>[2x]MALDLTGYLDRINYRGATDPTLDVLRDLVSAH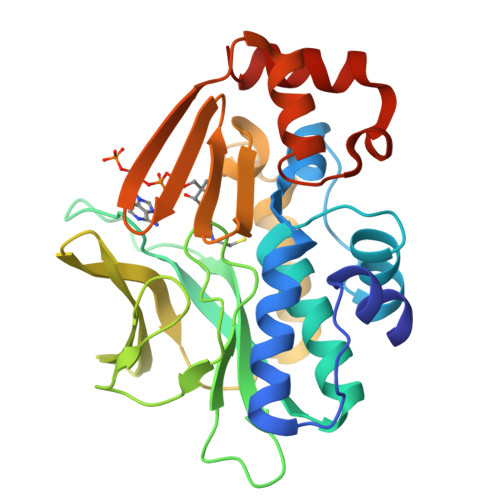TGAIAFENLDPLMGVPVDDLSAEALADKLVDRRRGGYCYEHNGLIGYVLAELGYRVRRLAGRVVWLAPPDAPTPAQTHTVLAVTFPGCQGPYLVDVGFGGMTPTAPLRLETGTVQQTALEPYRLDDRGDGLVLQAMVRDEWQALYEFSTLTRPQVDLRVGSWFVSTHPTSHFVTGLMAATVADDARWNLMGRNLAIHRRGGTEKILLEDAAAVVDTLGDRFGINVADVGERGRLEARIDKVCFGAENR>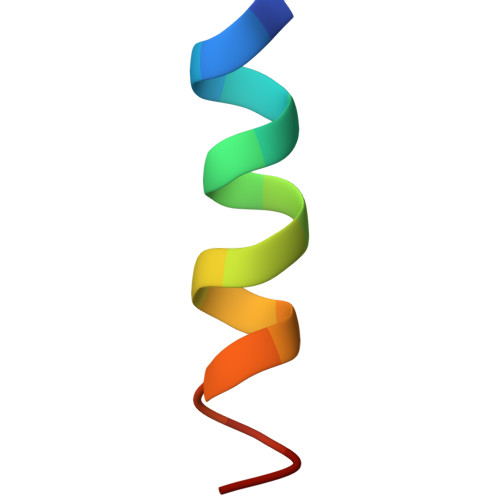 AALALAAAAALALAAAG>[5x]NAMIIRPEQHWFLRLFDWHGSVLSKIIFRLLLNVLMSIIAIISYQWYEQLGIHLTVAPFSLLGIAIAIFLGFRNSASYSRFVEARNLWGTVLIAERTLVRQLRNILPAEHDAHRRIVSYLVAFSWSLKHQLRKTDPTADLRRLLPEERVTEI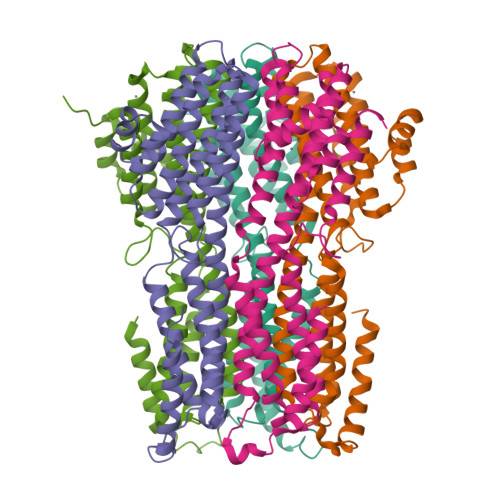LASSMPTNRILLLAGNEIGQLREAGKLSDITYGLMDNKLDELAHVLGGCERLATTPVPFAYTLILQRTVYLFCTLLPFALVGDLHYMTPFVSVFISYTFLSWDSLAEELEDPFGTAANALPLNAMCNTIERNLLDMTGQHPLPE>MDKTTFRLLRGESNLFYTLAKWENNKISVELPENLDMQSPTMTLIYDETGKLLWTQRNIPCLIKSIQPEWLKTNGFHEIETNVDCTSTLLSEDHSAQEKLKEVREDDDDAEMTHSVAVNIYPATARMPQL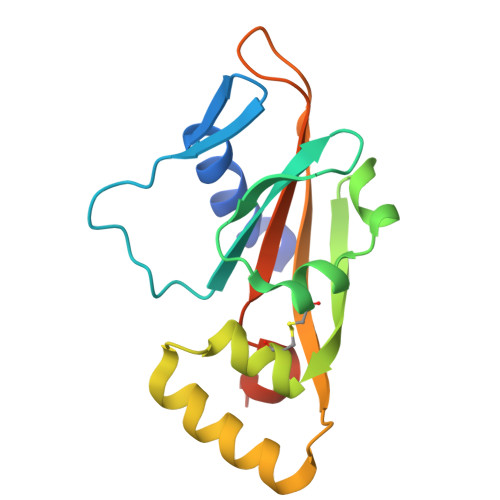TIVVVDTIPIELKRSYMHHHHHH[3x]>MVTALSDVNNTDNYGAGQIQVLEGLEAARKRPGMYIGSTSERGLHHLVWEIVDNSIDEALAGYANQIEVVIEKDNWIKVTDNGRGIPVDIQEKMGRPAVEVILTVLHAGGKFGGGGYKVSGGLHGVGSSVVNALSQDLEVYVHRNETIYHQAYKKGVPQFDLKEVGTTDKTGTVIRFKADGEI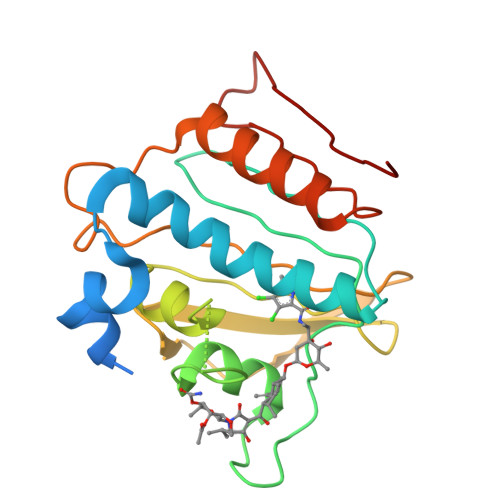FTETTVYNYETLQQRIRELAFLNKGIQITLRDERDEENVREDSYHYEG[4x]> MAFHWCDNNLHTTVFTPRDFQVELLATAYERNTIICLGHRSSKEFIALKLLQELSRRARRHGRVSVYLSCEVGTSTEPCSIYTMLTHLTDLRVWQEQPDMQIPFDHCWTDYHVSILRPEGFLYLLETRELLLSRVELIVLEDCHDSAVYQRIRPLFENHIMPAPPADRPRILGLAGPLHSAGCELQQLSAMLATLEQSVLCQIESASDIVTVLRYCSRPHEYIVQCAPFEMDELSLVLADVLNTHKSFLLDHRYDPYEIYGTDQFMDELKDIPDPKVDPLNVINSLLVVLHEMGPWCTQRAAHHFYQCNEKLKVKTPHERHYLLYCLVSTALIQLYSLCEHAFHRHLGSGSDSRQTIERYSSPKVRRLLQTLRCFKPEEVHTQADGLRRMRHQVDQADFNRLSHTLESKCRMVDQLDQPPTETRALVATLEQILHTTEDRQTNRSAARVTPTPTPAHAKPKPSSGANTAQPRTRRRVYTRRHHRDHNDGSDTLCALIYCNQNHTARVLFELLAEISRRDPDLKFLRCQYTTDRVADPTTEPKEAEL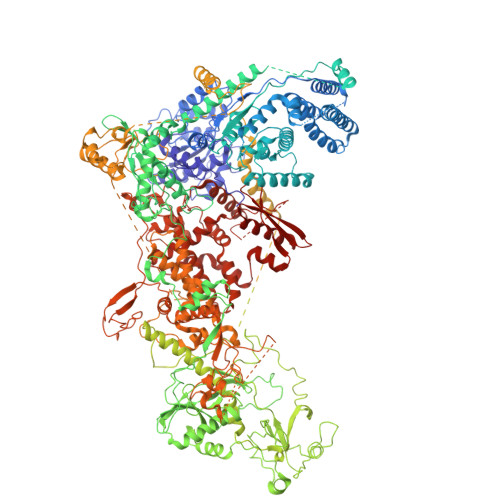EHRRQEEVLKRFRMHDCNVLIGTSVLEEGIDVPKCNLVVRWDPPTTYRSYVQCKGRARAAPAYHVILVAPSYKSPTVGSVQLTDRSHRYICATGDTTEADSDSDDSAMPNSSGSDPYTFGTARGTVKILNPEVFSKQPPTACDIKLQEIQDELPASAQLDTSNSSDEAVSMSNTSPSESSTEQKSRRFQCELSSLTEPEDTSDTTAEIDTAHSLASTTKDLVHQMAQYREIEQMLLSKCANTEPPEQEQCEAERFSACLAAYRPKPHLLTGASVDLGSAIALVNKYCARLPSDTFTKLTALWRCTRNERAGVTLFQYTLRLPINSPLKHDIVGLPMPTQTLARRLAALQACVELHRIGELDDQLQPIGKEGFRALEPDWECFELEPEDEQIVQLSDEPRPGTTKRRQYYYKRIASEFCDCRPVAGAPCYLYFIQLTLQCPIPEEQNTRGRKIYPPEDAQQGFGILTTKRIPKLSAFSIFTRSGEVKVSLELAKERVILTSEQIVCINGFLNYTFTNVLRLQKFLMLFDPDSTENCVFIVPTVKAPAGGKHIDWQFLELIQANGNTMPRAVPDEERQAQPFDPQRFQDAVVMPWYRNQDQPQYFYVAEICPHLSPLSCFPGDNYRTFKHYYLVKYGLTIQNTSQPLLDVDHTSARLNFLTPRYVNRKGVALPTSSEETKRAKRENLEQKQILVPELCTVHPFPASLWRTAVCLPCILYRINGLLLADDIRKQVSADLGLGRQQIEDEDFEWPMLDFGWSLSEVLKKSRESKQKESLKDDTINGKDLVDVEKKAISEETQIDKDSKDDKVEKSAIELIIEGEEKLQEADDFIEIGTWSNDMADDIASFNQEDDDEDDAFHLPVLPANVKFCDQQTRYGSPTFWDVSNGESGFKGPKSSQNKQGGKGKAKGPAKPTFNYYDSDNSLGSSYDDDDNAGPLNYMHHNYSSDDDDVADDIDAGRIAFTSKNEAETIETAQEVEKRQKQLSIIQATNANERQYQQTKNLLIGFNFKHEDQKEPATIRYEESIAKLKTEIESGGMLVPHDQQLVLKRSDAAEAQVAKVSMMELLKQLLPYVNEDVLAKKLGDRRELLLSDLVELNADWVARHEQETYNVMGCGDSFDNYNDHHRLNLDEKQLKLQYERIEIEPPTSTKAITSAILPAGFSFDRQPDLVGHPGPSPSIILQALTMSNANDGINLERLETIGDSFLKYAITTYLYITYENVHEGKLSHLRSKQVANLNLYRLGRRKRLGEYMIATKFEPHDNWLPPCYYVPKELEKALIEAKIPTHHWKLADLLDIKNLSSVQICEMVREKADALGLEQNGGAQNGQLDDSNDSCNDFSCFIPYNLVSQHSIPDKSIADCVEALIGAYLIECGPRGALLFMAWLGVRVLPITRQLDGGNQEQRIPGSTKPNAENVVTVYGAWPTPRSPLLHFAPNATEELDQLLSGFEEFEESLGYKFRDRSYLLQAMTHASYTPNRLTDCYQRLEFLGDAVLDYLITRHLYEDPRQHSPGALTDLRSALVNNTIFASLAVRHGFHKFFRHLSPGLNDVIDRFVRIQQENGHCISEEYYLLSEEECDDAEDVEVPKALGDVFESIAGAIFLDSNMSLDVVWHVYSNMMSPEIEQFSNSVPKSPIRELLELEPETAKFGKPEKLADGRRVRVTVDVFCKGTFRGIGRNYRIAKCTAAKCALRQLKKQGLIAKKD>[8x]MNFIRNNRRALIQRMGLTVTKQICDDLF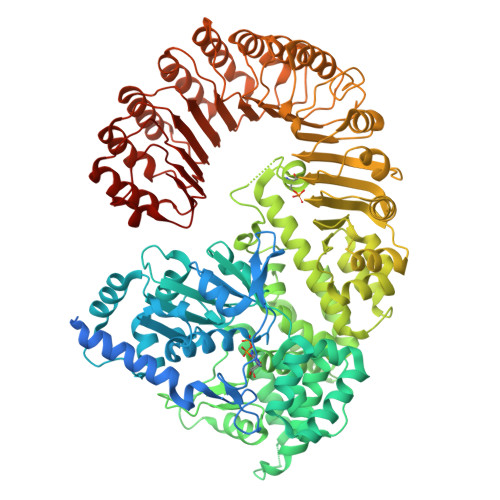ALNVLNNQEANVIYCEPLEQEAARKIIHMTMQKGSAACNLFLKSLENWDYFVYQDLTGQNLSYQVTEEDLNVLAQNLKDLYNSPAFLNFYPLGEDIDIIFNLEKTFTEPIMWKKDHRHHRVEQLTLGSLLEALKSPCLIEGESGKGKSTLLQRIAMLWASGGCRALKGFRLVFFIHLRSARGGLFETLYDQLLNIPDFISKPTFKALLLKLHKEVLFLLDGYNEFHPQNCPEIEALIKENHRFKNMVIVTTTTECLRHIRHVGALTAEVGDMTEDSAKDLIEAVLVPDQVERLWAQIQESRCLRNLMKTPLFVVITCAIQMGRQEFQAHTQTMLFQTFYDLLIQKNSHRYRGGASGDFARSLDYCGDLALEGVFAHKFDFEPEHGSSMNEDVLVTIGLLCKYTAQRLKPTYKFFHKSFQEYTAGRRLSSLLTSKEPEEVSKGNSYLNKMVSISDITSLYGNLLLYTCGSSTEATRAVMRHLAMVYQHGSLQGLSVTKRPLWRQESIQSLRNTTEQDVLKAINVNSFVECGINLFSESMSKSDLSQEFEAFFQGKSLYINSENIPDYLFDFFEYLPNCASALDFVKLDFYERATESQDKAEENVPGVHTEGPSETYIPPRAVSLFFNWKQEFKTLEVTLRDINKLNKQDIKYLGKIFSSATNLRLHIKRCAAMAGRLSSVLRTCKNMHTLMVEASPLTTDDEQYITSVTGLQNLSIHRLHTQQLPGGLIDSLGNLKNLERLILDDIRMNEEDAKNLAEGLRSLKKMRLLHLTHLSDIGEGMDYIVKSLSEESCDLQEMKLVACCLTANSVKVLAQNLHNLIKLSILDISENYLEKDGNEALQELIGRLGVLGELTTLMLPWCWDVHTSLPKLLKQLEGTPGLAKLGLKNWRLRDEEIKSLGEFLEMNPLRDLQQLDLAGHCVSSDGWLYFMNVFENLKQLVFFDFSTEEFLPDAALVRKLSQVLSKLTLLQEVKLTGWEFDDYDISAIKGTFKLVTA> MKPVTLYDVAEYAGVSYQTVSRVVNQASHVSAKTREKVEAAMAELNYIPNRVAQQLAGKQSLLIGVATSSLALHAPSQIVAAIKSRADQLGASVVVSMVERSGVEACKTAVHNLLAQRVSGLIINYPLDDQDAIAVEAACTNVPALFLDVSDQTPINSIIFSHEDGTRLGVEHLVALGHQQIALLAGPLSSVSARLRLAGWHKYLTRNQIQPIAEREGDWSAMSGFQQTMQMLNEGIVPTAMLVANDQMALGAMRAITESGLRVGADISVVGYDDTEDSSCYIPPLTTIKQDFRLLGQTSVDRLLQLSQGQAVKGNQLLPVS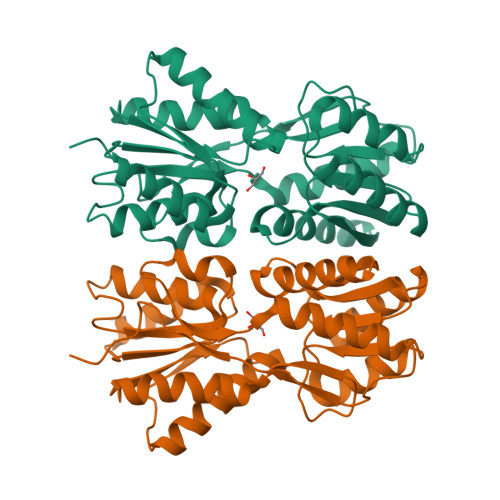LVKRKTTLAPNTQTASPRALADSLMQL>[2x]GSSMVTGGMASKWDQKGMDIAYEEALLGYKEGGVPIGGCLINNKDGSVLGRGHNMRFQKG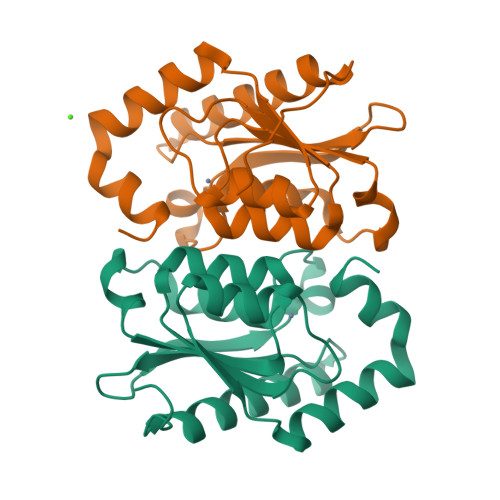SATLHGEISTLENCGRLEGKVYKDTTLYTTLSPCDMCTGAIIMYGIPRCVIGENVNFKSKGEKYLQTRGHEVVVVDDERCKKLMKQFIDERPQDWFEDIGE>[2x]SNAQDVPVTQVMTPRPVVFRVDATMTINEFLDKHKDTPFSRPL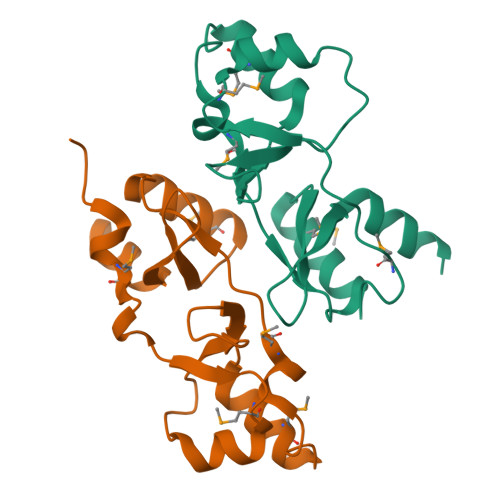VYSEQKDNIIGFVHRLELFKMQQSGSGQKQLGAVMRPIQVVLNNTALPKVFDQMMTHRLQLALVVDEYGTVLGLVTLEDIFEHLVGE>[3x]MAVLFADANQRGVHKHIFESDADVGADIAFNATPRSMVVLSGVWRLYRE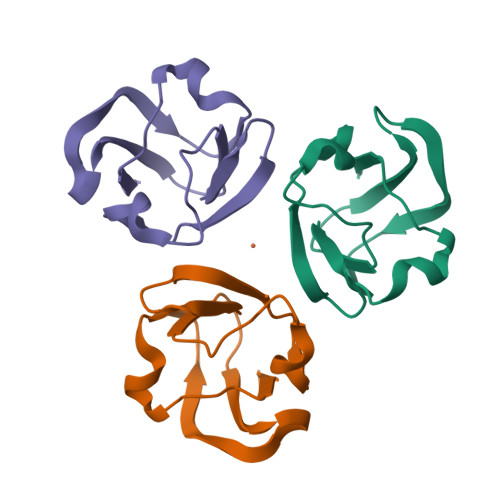PNFQSPYEAEFGPGIYPSIADYGINVIGSMKRIS> SMVRLKKSFGQHLLVSEGVLKKIAEELNIEEGNTVVEVGGGTGNLTKVLLQHPLKKLYVIELDREMVENLKSIGDERLEVINEDASKFPFCSLGKELKVVGNLPYNVASLIIENTVYNKD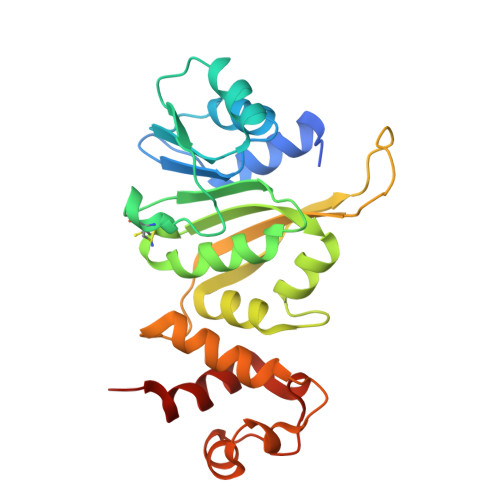CVPLAVFMVQKEVAEKLQGKKDTGWLSVFVRTFYDVNYVMTVPPRFFVPPPKVQSAVIKLVKNEKFPVKDLKNYKKFLTKIFQNRRKVLRKKIPEELLKEAGINPDARVEQLSLEDFFKLYRLIEDSGE Human prolyl‐hydroxylases 1‐3 (PHDs) are hypoxia‐sensing 2‐oxoglutarate (2OG) and FeII‐dependent oxygenases that regulate levels of the hypoxia‐inducible transcription factor α‐subunits (HIFα). The PHDs catalyse trans‐4‐prolyl hydroxylation of proline‐residues of the HIFα N‐ and C‐terminal oxygen degradation domains (NODD and CODD), reactions coupled to conversion of dioxygen and 2OG to succinate and carbon dioxide. Hydroxyproline formation promotes HIFα degradation through stabilisation of its interaction with the von Hippel‐Lindau (pVHL) protein‐E3 ligase complex resulting in HIFα ubiquitination and proteasomal proteolysis. PHD inhibition is a promising treatment of anaemia in chronic kidney disease by promotion of EPO‐mediated erythropoiesis and has potential to treat other ischaemia‐related disorders.

In the related compound IOX4, the morpholine ring of Molidustat is replaced with a tert‐butyl ester to enable brain penetration. Molidustat and IOX4 are potent inhibitors with reported half‐maximal inhibitory concentration (IC50) values of 7 and 3 nM, respectively, for isolated PHD2. The crystal form diffracted in the P21 space group with six PHD2181‐407 molecules in the asymmetric unit (ASU, chains A–F); PHD2 is principally monomeric in solution. Molidustat and IOX4, bind in a similar mode to the metal ion, that is, through bidentate chelation of their pyrimidine/pyridine N1 (2.15 Å/2.14 Å, trans to His374 NE2) and pyrazolone (2.27 Å/2.24 Å, trans to Asp315 OD1) nitrogens; the distance values reported here and subsequently are as observed in chain A of the PHD2‐Molidustat and PHD2‐IOX4 complex structures, respectively. Consistent with the established role of triazoles as carboxylate bioisosteres, those of Molidustat and IOX4 are located in a similar manner in the predominantly hydrophobic (except for Arg383 and Tyr329) 2OG C5 carboxylate binding pocket of PHD2. The triazoles do not make a H bond with Tyr‐303, instead π‐π stacking with this residue, which makes a H bond with the enolic form of the pyrazolone ring of Molidustat/IOX4. The structures imply that both Molidustat and IOX4 probably bind at the active site with their pyrazolone ring (at least) predominantly in its enol form, as supported by the likely presence of a H bond between the enol and the phenol of Tyr303 (2.63 Å/2.71 Å) and metal ligation via the imine (N2) pyrazolone nitrogen. The Molidustat/IOX4 triazoles are positioned to π‐π stack with Tyr303 (3.55 Å/3.63 Å) and are perpendicular relative to Tyr310 (3.49 Å/3.51 Å); this interaction is not observed with the PHD2‐Vadadustat and FG‐2216 complexes. The Molidustat and IOX4 morpholine and tert‐butyl ester carboxylate side chains, respectively, extend out of the active site. The interaction between the tert‐butyl ester carbonyl of IOX4 and Arg322 may in part reflect the observation that IOX4 displaces HIF1α‐NODD more efficiently than Molidustat, though the details of how this occurs are unclear and may involve correlated motions.

>PNGQTKPLPALKLALEYIVPCMNKHGICVVDDFLGKETGQQIGDEVRALHDTGKFTDGQLVSQKSDSSKDIRGDKITWIEGKEPGCETIGLLMSSMDDLIRHCNGKLGSYKINGRTKAMVACYPGNGTGYVRHVDNPNGDGRCVTCIYYLNKDWDAKVSGGILRIFPEGKAQFADIEPKFDRLLFFWSDRRNPHEVQPAYATRYAITVWYFDADERARAKVKYLTGE[6x]>[6x]MSESINNITKPKERRDFVVMAGMRKDGTIDFIKVYALNEKLAIEVLEAFLKENNIHPSDFIVIQRGYEDVKDKKAITTRSEEELSAMLGRLGLRLVSNGVLYTDGIDKLYQITAISRELFESLQKEKREIFEDVQEKIT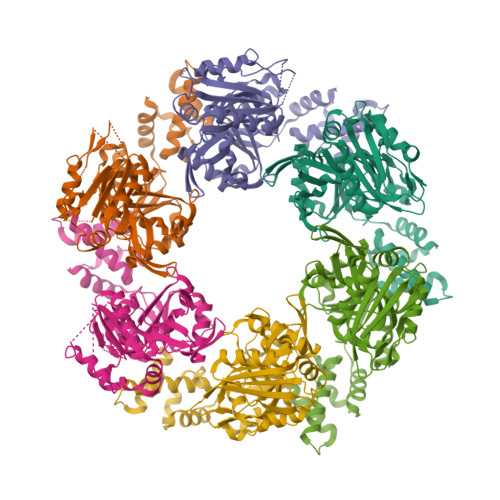FNFSKVDLPEKYVKKLRLLELMEDTIIFNMAELEIPNLLKAIVEGTVLIPRFLEKEDLIIRIFDEELHEYRGSYFDKVLIKPPIIHWDFYLDSLEDFSFKKVEESIYIAPLFLRATGGFLILTEPPEDLVKTLLKLKKRGEVRTILEGKRITIPINFTLIVDTRHPERYAGLKFPIRINLPPLDDETFLKVLETNLGITPPTEIVRIFPPDYKTFLGVELIKNLFEKLKLTEKGKDEVSLLKEAATIITGGTPGGSSGGSGHHHHHH5-bromo-N-(diphenylmethyl)-N-methylthiophene-2-carboxamide | C19 H16 Br N O S 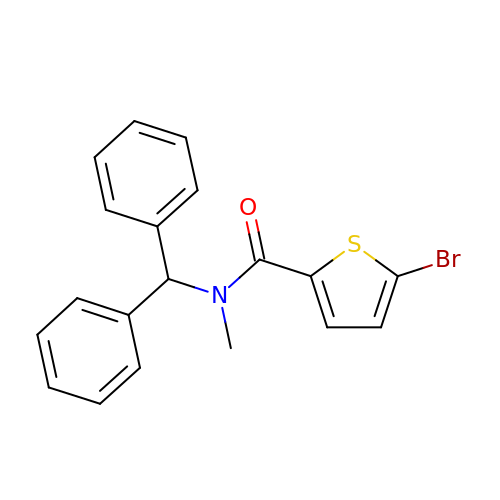| WORZHUYQQIIZTA-UHFFFAOYSA-N> MAKIGL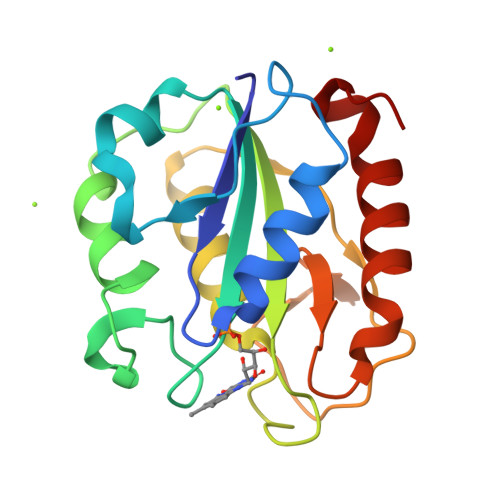FFGSNTGKTRKVAKSIKKRFDDETMSDALNVNRVSAEDFAQYQFLILGTPTLGEGELPGLSSDCENESWEEFLPKIEGLDFSGKTVALFGLGDQVGYPENYLDALGELYSFFKDRGAKIVGSWSTDGYEFESSEAVVDGKFVGLALDLDNQSGKTDERVAAWLAQIAPEFGLSL> MARFFIDRPVFAWVISLLIVLAGVLAIRFLPVAQYPDIAPPVVNVSASYPGASAKVVEEAVTAIIEREMNGAPGLL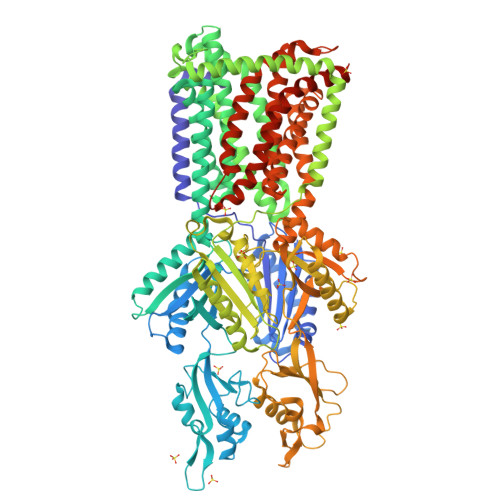YTKATSSTGQASLTLTFRQGVNADLAAVEVQNRLKIVESRLPESVRRDGIYVEKAADSIQLIVTLTSSSGRYDAMELGEIASSNVLQALRRVEGVGKVETWGAEYAMRIWPDPAKLTSMNLSASDLVNAVRRHNARLTVGDIGNLGVPDSAPISATVKVDDTLVTPEQFGEIPLRIRADGGAIRLRDVARVEFGQSEYGFVSRVNQMTATGLAVKMAPGSNAVATAKRIRATLDELSRYFPEGVSYNIPYDTSAFVEISIRKVVSTLLEAMLLVFAVMYLFMQNFRATLIPTLVVPVALLGTFTVMLGLGFSINVLTMFGMVLAIGILVDDAIIVVENVERLMAEEGLSPHDATVKAMRQISGAIVGITVVLVSVFVPMAFFSGAVGNIYRQFAVTLAVSIGFSAFLALSLTPALCATLLRPIDADHHEKRGFFGWFNRAFLRLTGRYRNAVAGILARPIRWMLVYTLVIGVVALLFVRLPQAFLPEEDQGDFMIMVMQPEGTPMAETMANVGDVERYLAEHEPVAYAYAVGGFSLYGDGTSSAMIFATLKDWSERREASQHVGAIVERINQRFAGLPNRTVYAMNSPPLPDLGSTSGFDFRLQDRGGVGYEALVKARDQLLARAAEDPRLANVMFAGQGEAPQIRLDIDRRKAETLGVSMDEINTTLAVMFGSDYIGDFMHGSQVRKVVVQADGAKRLGIDDIGRLHVRNEQGEMVPLATFAKAAWTLGPPQLTRYNGYPSFNLEGQAAPGYSSGEAMQAMEQLMQGLPEGIAHEWSGQSFEERLSGAQAPALFALSVLIVFLALAALYESWSIPLAVILVVPLGVLGALLGVSLRGLPNDIYFKVGLITIIGLSAKNAILIIEVAKDHYQEGMSLLQATLEAARLRLRPIVMTSLAFGFGVVPLALSSGAGSGAQVAIGTGVLGGIVTATVLAVFLVPLFFLVVGRLFRLRKAPRTGNSPQIPTEQAHHHHHHHHH Nitrogenases catalyze a key step in the global nitrogen cycle by reducing molecular nitrogen (dinitrogen, N2) to ammonia (NH3). Some diazotrophs encode ‘back-up’ or alternative nitrogenase genes: vnfHDGK for the vanadium (V) nitrogenase or anfHDGK for the iron (Fe) nitrogenase, expressed upon the depletion of Mo. Upon complex formation, low-potential electrons are transferred from the [Fe4S4] cluster of the reductase component via an [Fe8S7] relay (P-cluster) to the active site cofactor of the catalytic component. The active site cofactor is expected to follow the general composition of [MFe7S9C-(R)-homocitrate], where M is Mo, V or Fe, depending on the nitrogenase isoform.

To examine if the αIII domain flexibility is observed or even amplified in the resting state of the catalytic component, we tried to solve the cryo-EM structure of Anf(DGK)2. Using identical conditions as for the AlF3-trapped complex, particle orientation had a strong bias for top views on AnfD. To circumvent the preferred orientation problem, we collected another data set of the catalytic component with CHAPSO detergent added right before plunge freezing of the grids. The use of detergent mitigated the preferred orientation problem, and we obtained a cryo-EM map with a global resolution of 2.49 Å. However, the map is missing electron density for AnfG, suggesting that it was solubilized from the complex after the addition of CHAPSO. In support of this hypothesis, loss of AnfG after the addition of detergent leads to a destabilization of the αIII domain accompanied by the loss of the FeFeco. Thus, the G subunit might stabilize the active site cofactor through interaction with the αIII domain.

>[2x]MPYHEFEVSKCIPERREHAVMKAAGEDLTSCLPKGYLNTIPGTISERGCAYCGAKHVIGTPMKDVIHISHGPNGCTYDTWQTKRYISDNDNFQLKYTFATDVKEKHVVFGAEGLLKKSMHEAFDAFPNIKRMTVYQTCTTALIGDDVDAIAKEVMEERGDVDVFVCNSPGFAGPSQSGGHHKINIAWLNQKVGTVEPDYLGEHVINYVGEYNIQGDQEVMIDYFNRMGIQVLSTFTGNGSYDSLRMMHRAHLNVLECARSAEYICDELRARYGIPRLDIDGFGFEPLANSLRKVALFFGIEDKAEAIIAEEYAKWKPQLDWYKERLKGKKVCLWPGGSKLWHWAHAIEEEMGLKVVSVYTKFGHQGDMEKGVSRCGEGALAIDDPNELESVEAIEMLKPDIIFTGKRPGEFVKKHGVPYLNAHAYHNGPYKGFEGWVRFARDIYNAIYSPMRQLAALDISAPDAAITSGFRTAKMNADLTVSDEVKFSEVLHEYTGKYDSIAEIRARNQAYAAEQKALRDAVQPAAEWSHPQFEK;>MTCQVTQKAREGTINPIFTCQPAGAQFASIGIKDCIGIVHGGQGCVMFVRLLISQHMKESFEIASSSVHEDGAVFGALDRVETAVEVLLTRYPDVKVVPIITTCSTEIIGDDVDGLLSKLEDELLPTKFPGREVHLLTVHCPSFVGSMITGYDKAVHDFVKKFATKDEPSDKINLITGWVNPGDVKELKHLLEVMEVKANVLFEVESFDSPLMPDLEHHSHGSTTIEDLRDTANAKGTIALNRYEGMKAADYLKKKFKVPAVIGPTPVGIRNTDAFLKAVSEMTGQPIPAQLVKERGLALDAIADIGHMFLADKRVAIYANPDLAIGLTEFCLDLEMKPKLLLLGDDNSGYVKDPRVLALQENAPDLEIVTNADFWDLESRIQQGLELDLILGHSKGRFISIDYKVPMVRVGFPTYDRAGMYRHPVLGYGGAMFLAETMANTLFADMEAKKNKEWILNVW[2x]>[6x]GANFQYIITEKKGKNSSVGLIQLNRPKALNALCNGLIEELNQALETFEEDPAVGAIVLTGGEKAFAAGADIKEMQNRTFQDCYSGKFL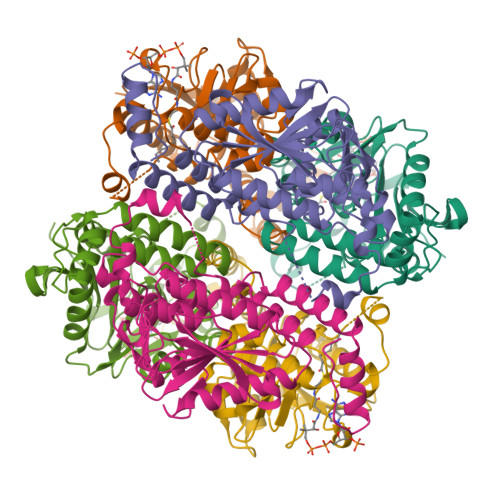SHWDHITRIKKPVIAAVNGYALGGGCELAMMCDIIYAGEKAQFGQPEILLGTIPGAGGTQRLTRAVGKSLAMEMVLTGDRISAQDAKQAGLVSKIFPVETLVEEAIQCAEKIANNSKIIVAMAKESVNAAFEMTLTEGNKLEKKLFYSTFATDDRREGMSAFVEKRKANFKDH> MTADELVFFVNGKKVVEKNADPETTLLVYLRRKLGLCGTKLGCGEGGCGACTVMISKYDRLQNKIVHFSVNACLAPICSLHHVAVTTVEGIGNTQKLHPVQERIARSHGSQCGFCTPGIVMSMYTLLRNQPEPTVEEIENAFQGNLCRCTGYRPILQGFRTFAKDGGCCGGSGNNPNCCMNQTKDQTVSLSPSLFNPEDFKPLDPTQEPIFPPELLRLKDTPQKKLRFEGERVTWIQASTMEELLDLKAQHPDAKLVVGNTEIGIEMKFKNMLFPLIVCPAWIPELNSVVHGPEGISFGASCPLSLVESVLAEEIAKLPEQKTEVFRGVMEQLRWFAGKQVKSVASIGGNIITASPISDLNPVFMASGAKLTLVSRGTRRTVRMDHTFFPGYRKTLLRPEEILLSIEIPYSKEGEFFSAFKQASRREDDIAKVTSGMRVLFKPGTIEVQELSLCFGGMADRTISALKTTPKQLSKSWNEELLQSVCAGLAEELQLAPDAPGGMVEFRRTLTLSFFFKFYLTVLQKLGRADLEDMAGKLDPTFASATLLFQKDPPANVQLFQEVPKDQSEEDMVGRPLPHLAANMQASGE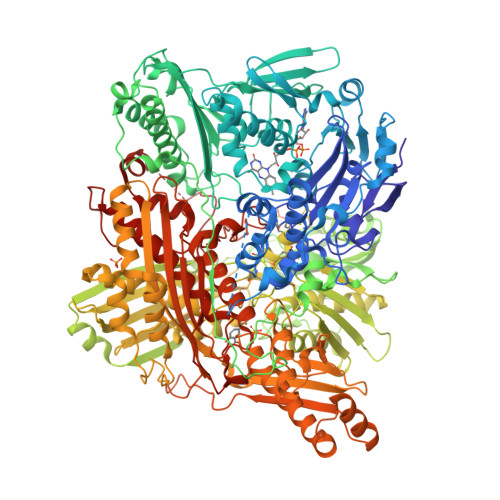AVYCDDIPRYENELSLRLVTSTRAHAKITSIDTSEAKKVPGFVCFLTAEDVPNSNATGLFNDETVFAKDEVTCVGHIIGAVVADTPEHAQRAARGVKITYEDLPAIITIQDAINNNSFYGSEIKIEKGDLKKGFSEADNVVSGELYIGGQEHFYLETNCTIAVPKGEAGEMELFVSTQNTMKTQSFVAKMLGVPDNRIVVRVKRMGGGFGGKETRSTVVSTALALAAHKTGRPVRCMLDRDEDMLITGGRHPFLAKYKVGFMKTGTVVALEVAHFSNGGNTEDLSRSIMERALFHMDNAYKIPNIRGTGRICKTNLPSNTAFRGFGGPQGMLIAEYWMSEVAITCGLPAEEVRRKNMYKEGDLTHFNQKLEGFTLPRCWDECIASSQYLARKREVEKFNRENRWKKRGLCIIPTKFGISFTLPFLNQGGALVHVYTDGSVLLTHGGTEMGQGLHTKMVQVASRALKIPTSKIHISETSTNTVPNTSPTAASASADLNGQGVYEACQTILKRLEPFKKKKPTGPWEAWVMDAYTSAVSLSATGFYKTPNLGYSFETNSGNPFHYFSYGVACSEVEIDCLTGDHKNLRTDIVMDVGSSLNPAIDIGQVEGAFVQGLGLFTMEELHYSPEGSLHTRGPSTYKIPAFGSIPIEFRVSLLRDCPNKRAIYASKAVGEPPLFLASSIFFAIKDAIRAARAQHGDNAKQLFQLDSPATPEKIRNACVDQFTTLCVTGVPENSKSWSVRI>[2x]MSRLDKSKVINSALELLNEVGIEGLTTRKLAQKLGVEQPTLYWHVKNKRALLDALAIEMLDRHHT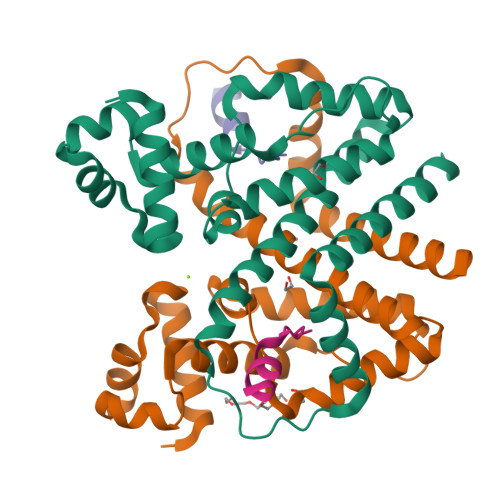HFSPLEGESWQDFLRNNAKSFRNALLSHRDGAKVHLGTRPTEKQYETLENQLAFLTQQGFSLENALYALSAVGHFTLGSVLEDQEHQVAKEERETPTTDSMPPLLRQAIELFDHQGAEPAFLHGLESLIRGFEVQLTALLQIV;>[2x]DDSVLAARARMWMWHW> AETVESCLAKPHTENSFTNVWKDDKTLDRYANYEGCLWNATGVVVCTGDETQCYGTWVPIGLAIPENEGGGSEGGGSEGGGSEGGGTKPPEYGDTPIPGYTYINPLDGTYPPGTEQNPANPNPSLEESQPLNTFMFQNNRFRNRQGALTVYTGTVTQGTDPVKTYYQYTPVSSKAMYDAYWNGKFRDCAFHSGFNEDPFVCEYQGQSSDLPQPPVNAGGGSGGGSGGGSEGGGSEGGGSEGGGSEGGGSGGGSGSGDFDYEKMANANKGAMTENADENALQSDAKGKLDSVATDYGAAIDGFIGDVSGLANGNGATGDFAGSNSQMAQVGDGDNSPLMNNFRQYLPSLPQSVECRPFVFGAGKPYEFSIDCDKINLFRGVFAFLLYVATF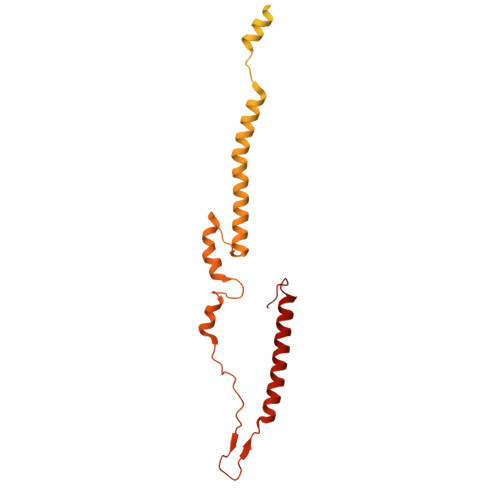MYVFSTFANILRNKES>[4x]MRGSHHHHHHGSAEPPNMPSMAPVLKNIMPAIVNVAVQGYLPN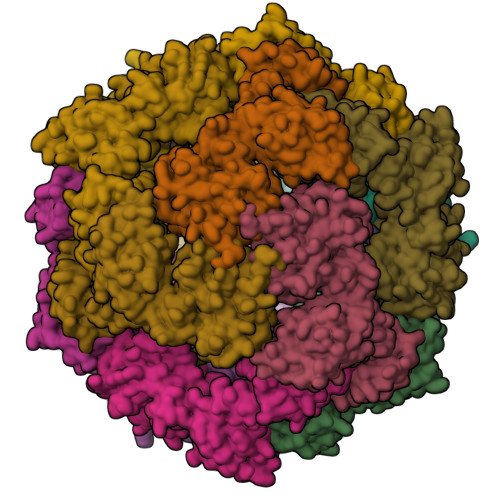DVTPPGSAGNDEENQPNNRPPQSRMPEKGRKFESIGSGVIIDPNNGVIITNDHVIRNASLITVTLQDGRRLKARLIGGDSETDLAVLKIDAKNLKSLVIGDSDKLEVGDFVVAIGNPFGLNSFGNSQSATFGIVSALKRSDLNIEGVENFIQTDAAINPGNAGGALVNAKGELIGINTAILSPYGGNVGIGFAIPINMVKDVAQQIIKFGSIHRGLMGIFVQHLTPELAQAMGYPEDFQGALVSQVNPNSPAELAGLKAGDIITQINDTKITQATQVKTTISLLRVGSTVKIIVERDNKPLTLSAVVTDIKSHEQKLQSNNPFLYGLALRAFEQESPPHGNVIGVQVVGASENSAGWRAGIRPGDIIISANKKPVTDVKSLQTIAQEKKKELLVQVLRGPGSMYLLVI>[4x]MAPIEWESSPRVEVFVGRKRELSIIRNAKGVVVIYGIAGIGKTSLAAKAFPNAYWYNVTGLEDFKYFAWQLGLFLSSIGFEDLLE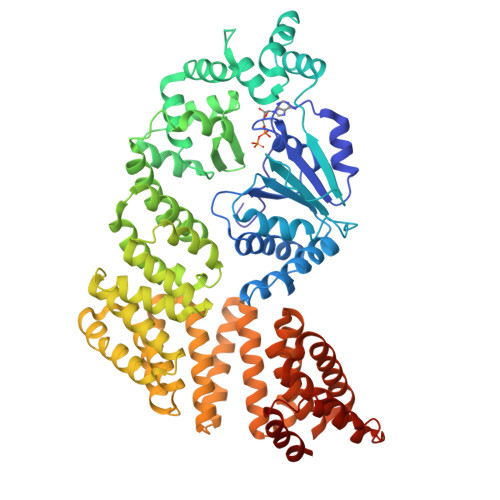YLRGGGNNENDIFKLITEGIEKTGAIIIIDDFHKFQDEKVNYLLSYLAPRIKKGKVIITTRIRPNLGNEGVTYVNLKGLNPEEAYSLAREKEKSMTPEEFAKLYKLTFGHPLMLNLILESSEILATGKDTVFNFLFEEVYQMLNEEEKDLLSILSLFDEPIEYEGIKFLYDRNPFVPLYSLMKKGLIEKKGEKYFVHDMVREFVREVSNQEEKEVYLRHVNFLLKSKTPINFLRAFKYAIKVGSSELIRNLVELRVKEFYRIIVDFPRMYQRLLMEVEDNPYAKIEIAIIEVQRGLFEKAIKLLKEAEPYVDEFFKCEIYSWLADAYMELENLEKAERYLKKTKEIVEKINDMYAWFSYYAEKTKYEYYKENSREALKSALKELEIIRKIGDPEKEGLVLLHVGDIYLHMGNYEKGISYYQEALKMAKAYGIKFLEHISYMELAKGYYQLKLYEKASEYSEKAANYFLMIRNYRRATDAMAYGSVSYIATKNLEKAEKFAKEMIRIAQSTDYPLAWAGYIFLAAVDFLKGDDWREDYNLGKAHLKEYPWLFEAVLDELKKVFDLSNFK> ATYSTVPKIAFYAGLKRQHEGYEVLKFDDVVTNLGNHYDPT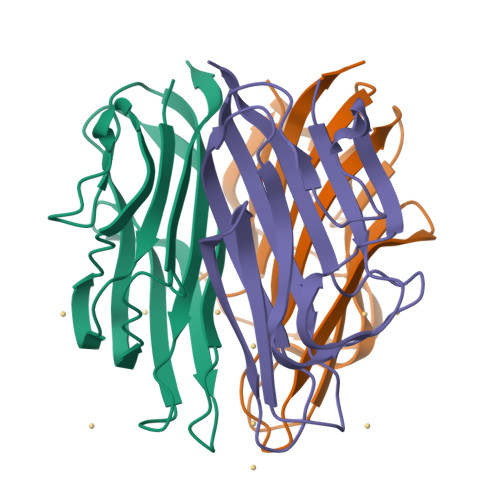TGKFTCSIPGIYFFTYHVLMRGGDGTSMWADLCKNNQVRASAIAQDADQNYDYASNSVVLHLEPGDEVYIKLDGGKAHGGNNNKYSTFSGFIIYAD>[2x]SANVTQAFGRRGPEQT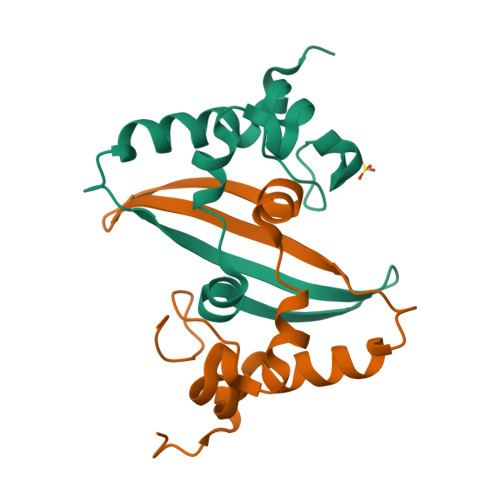QGNFGDQDLIRQGTDYKHWPQIAQFAPSASAFFGMSRIGMEVTPSGTWLTYHGAIKLDDKDPQFKDNVILLNKHIDAYKTFPPTEPK> MKCLVTGGNVKVLGKAVHSLSRIGDELYLEPLEDGLSLRTVNSSRSAYACFLFAPLFFQQYQAATPGQDLLRCKILMKSFLSVFRSLAMLEKTVEKCCISLNGRSSRLVVQLHCKFGVRKTHNLSFQDCESLQAVFDPASCPHMLRAPARVLGEAVLPFSPALAEVTLGIGRGRRVILRSYHEEEADSTAKAMVTEMCLGEEDFQQLQAQEGVAITFCLKEFRGLLSFAESANLNLSIHFDAPGRPAIFTIKDSLLDGHFVLATLSDTDS;> MHHHHH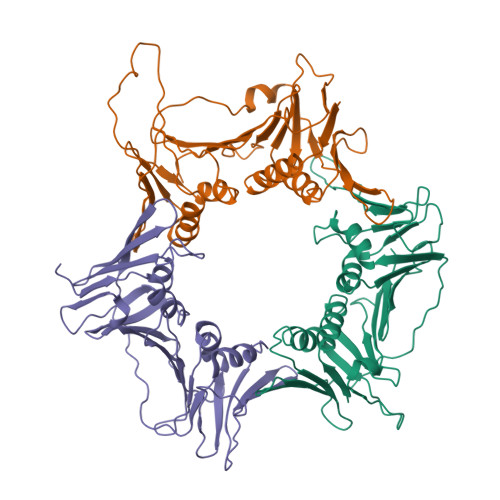HKFRAKIVDGACLNHFTRISNMIAKLAKTCTLRISPDKLNFILCDKLANGGVSMWCELEQENFFNEFQMEGVSAENNEIYLELTSENLSRALKTAQNARALKIKLTNKHFPCLTVSVELLSMSSSSRIVTHDIPIKVIPRKLWKDLQEPVVPDPDVSIYLPVLKTMKSVVEKMKNISNHLVIEANLDGELNLKIETELVCVTTHFKDLGNPPLASESTHEDRNVEHMAEVHIDIRKLLQFLAGQQVNPTKALCNIVNNKMVHFDLLHEDVSLQYFIPALS;> MPLLTQQIQDEDDQYSLVASLDNVRNLSTILKAIHFREHATCFATKNGIKVTVENAKCVQANAFIQAGIFQEFKVQEESVTFRINLTVLLDCLSIFGSSPMPGTLTALRMCYQGYGYPLMLFLEEGGVVTVCKINTQEPEETLDFDFCSTNVINKIILQSEGLREAFSELDMTSEVLQITMSPDKPYFRLSTFGNAGSSHLDYPKDSDLMEAFHCNQTQVNRYKISLLKPSTKALVLSCKVSIRTDNRGFLSLQYMIRNEDGQICFVEYYCCPDEEVPESES4-[(2-methyl-3,4-dihydro-1~{H}-pyrido[4,3-b]indol-5-yl)methyl]-~{N}-oxidanyl-benzamide 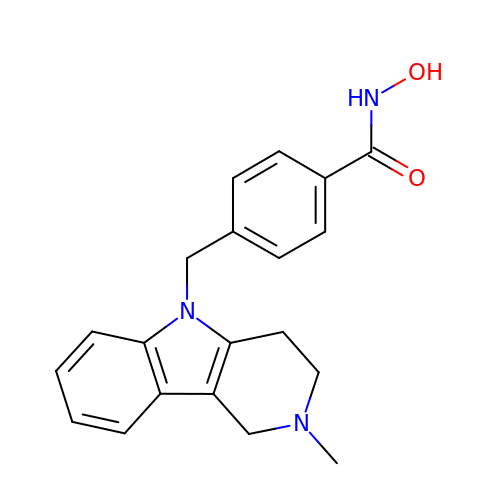| C20 H21 N3 O2 | GOVYBPLHWIEHEJ-UHFFFAOYSA-N> SEFENPLKRLLVPGEEWEFEVTAFYRGRQVFQQTISCPEGLRLVGSEVGDRTLPGWPVTLPDPGMSLTDRGVMSYVRHVLS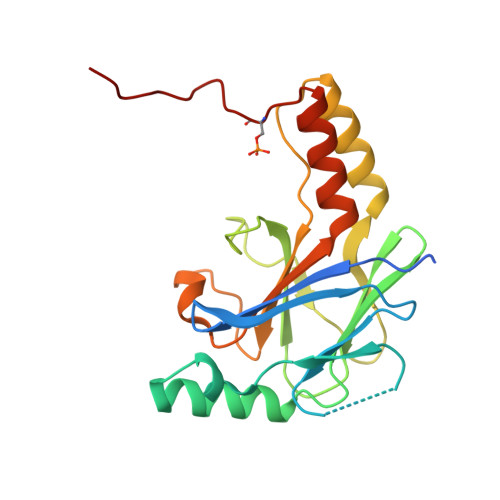CLGGGLALWRAGQWLWAQRLGHCHTYWAVSEELLPNSGHGPDGEVPKDKEGGVFDLGPFIVDLITFTEGSGRSPRYALWFCVGESWPQDQPWTKRLVMVKVVPTCLRALVEMARVGGASSLENTVDLHISNS6-ethyl-1H-pyrimidine-2,4-dione 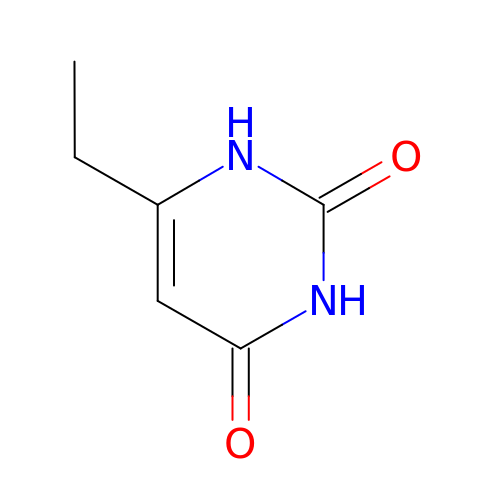| C6 H8 N2 O2 | JKUXMZDHLUUPGG-UHFFFAOYSA-N>[2x]PEFFSVRHLELAGDDPYSNVNCTKILQGDPEEIQKVKLEILTVQFKKRPRWTPHDYINMTRDCASFIRTRKYIVEPLTKEEVGFPIAYSIVVHHKIEMLDRLLRAIYMPQNFYCIHVDRKAEESFLAAVQGIASCFDNVFV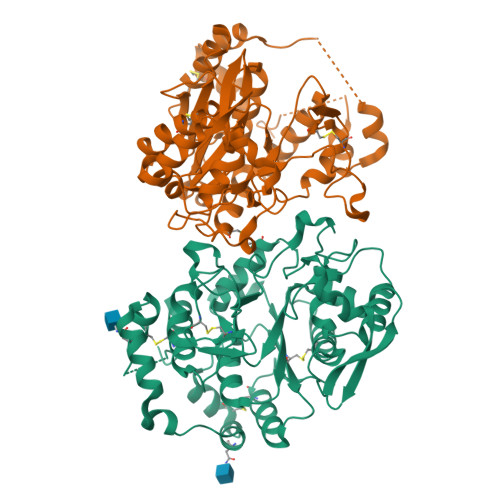ASQLESVVYASWTRVKADLNCMKDLYRMNANWKYLINLCGMDFPIKTNLEIVRKLKCSTGENNLETEKMPPNKEERWKKRYAVVDGKLTNTGIVKAPPPLKTPLFSGSAYFVVTREYVGYVLENENIQKLMEWAQDTYSPDEFLWATIQRIPEVPGSFPSSNKYDLSDMNAIARFVKWQYFEGDVSNGAPYPPCSGVHVRSVCVFGAGDLSWMLRQHHLFANKFDMDVDPFAIQCLDEHLRRKALENLEH>[2x]MKSNEHDDCQVTNPSTGHLFDLSSLSGRAGFTAAYSEKGLVYMSICGENENCPPGVGACFGQTRISVGKANKRLR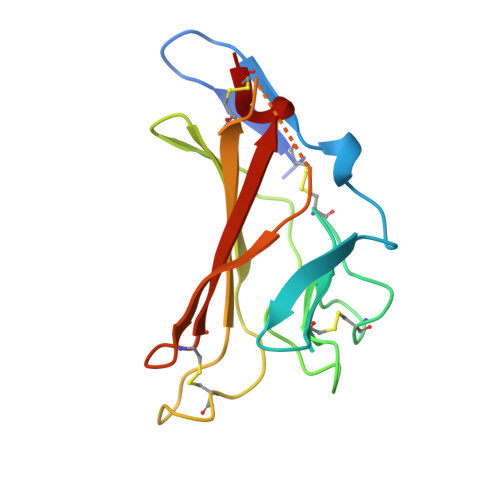YVDQVLQLVYKDGSPCPSKSGLSYKSVISFVCRPEAGPTNRPMLISLDKQTCTLFFSWHTPLACEQAT Here, selenomethionine derivatization and mercury soaking have been investigated for SFX experiments using the high-energy XFEL at the SPring-8 Angstrom Compact Free-Electron Laser (SACLA), Hyogo, Japan. Three successful cases are reported of single-wavelength anomalous diffraction (SAD) phasing using X-rays of less than 1 Å wavelength with reasonable numbers of diffraction patterns (13 000, 60 000 and 11 000). We succeeded in experimental phasing using SeMet-derivatization and Hg-soaking techniques at wavelengths of 0.954 and 0.984 Å, respectively. Such high-energy X-rays, which are essential for Se-SAD, allowed us to collect data at high resolution (1.4–1.6 Å) and perform SAD phasing with 11 000–60 000 indexed patterns.

SeMet-labeled ACG (Agrocybe cylindracea galectin) crystals belong to the space group P65 and have two monomers in the asymmetric unit. Each polypeptide consists of 178 residues and contains two Met residues; however, the first set of residues, including one Met residue, is disordered and the Bijvoet ratio is ∼2.2% at 13.0 keV. As the lattice symmetry (6/mmm) is higher than the Laue symmetry (6/m), there was a need to resolve the indexing ambiguity. The lower Bijvoet ratio and indexing ambiguity complicate the structure determination. Prior to merging using partialator, the twofold indexing ambiguity (hkl and ) was resolved using ambigator in the CrystFEL suite. We tested various numbers of patterns in the SAD phasing in the same way. At least 60 000 patterns (a mean multiplicity of 443.4 at 1.5 Å resolution) were required for SAD phase determination. The localization of Se sites required 35 000 patterns. The electron-density map from 60 000 patterns was readily interpretable. In the anomalous difference Fourier map, two Se sites with peak heights of 24.6σ and 24.1σ were identified. The number of patterns required for the ACG-Se case was much larger than others.

>[2x]MDYKDDDDKHMTTSAVNIYNISAGASVDLAAPVTTGDIVTFFSSALNLSAGAGSPNNTALNLLSENGAYLLHIAFRLQENVIVFNSRQPNAPWLVEQRVSNVANQFIGSGGKAMVTVFDHGDKYQVVINEKTVIQYTKQISGTTSSLSYNSTEGTSIFSTVVEAVTYTGLAKLAAALE~{N}-[(5~{S})-5-[[2,3-bis(oxidanyl)phenyl]carbonylamino]-6-oxidanylidene-6-(prop-2-ynylamino)hexyl]-2,3-bis(oxidanyl)benzamide 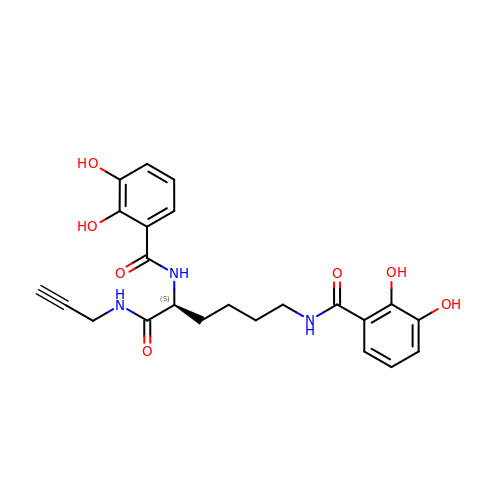| C23 H25 N3 O7 | PCGZMSMZUKWVQZ-INIZCTEOSA-N~{N}-[3-[6-azanyl-5-[2-[methyl(propanoyl)amino]ethoxy]pyrimidin-4-yl]-5-fluoranyl-2-methyl-phenyl]-4-cyclopropyl-2-fluoranyl-benzamide | C27 H29 F2 N5 O3 | 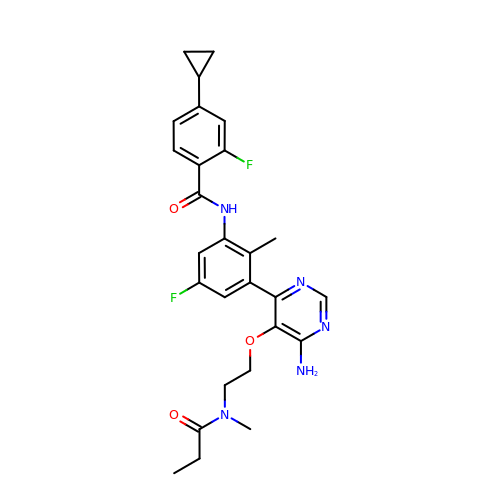CTBIYDHGUMTQNM-UHFFFAOYSA-N>GSHMARESAEEVWGGTEDLTSLSVEELKGLMARFDEEEKRISYRRRVMQGRIDVIRAEIVRRGGAV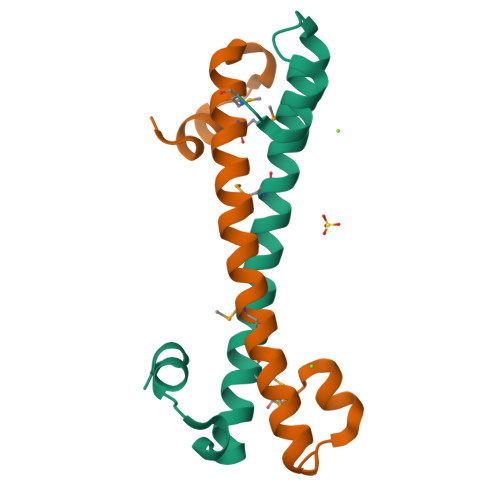LSPEELARVLMGDVGDESE[3x]(2S)-3-[(2E,6E)-3,7,11-trimethyldodeca-2,6,10-trienoxy]propane-1,2-diol | C18 H32 O3 | 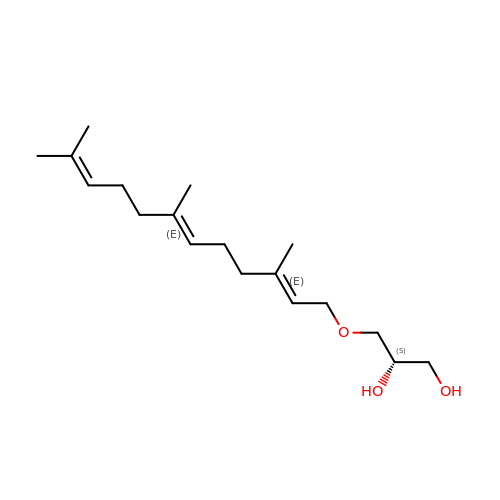VGIZXGYRSPTVQF-RNKQFFRGSA-N>[2x]MACEG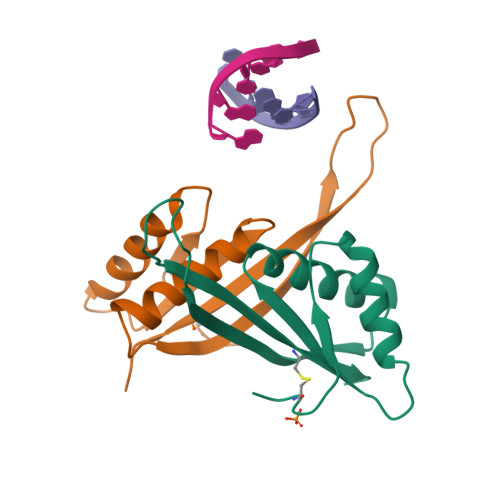APEVRIGRKPVMNYVLAILTTLMEQGTNQVVVKARGRNINRAVDAVEIVRKRFAKNIEIKDIKIDSQEIEVQTPEGQTRTRRVSSIEICLEKAGESA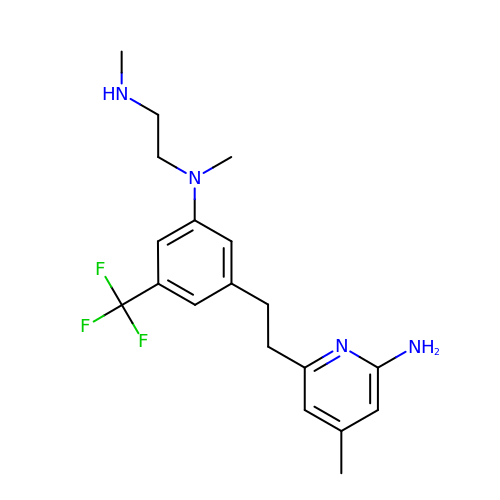N1-(3-(2-(6-AMINO-4-METHYLPYRIDIN-2-YL)ETHYL)-5-(TRIFLUOROMETHYL)PHENYL)-N1,N2-DIMETHYLETHANE-1,2-DIAMINE | C19 H25 F3 N4 | HEAUHZMVJKXAQR-UHFFFAOYSA-N>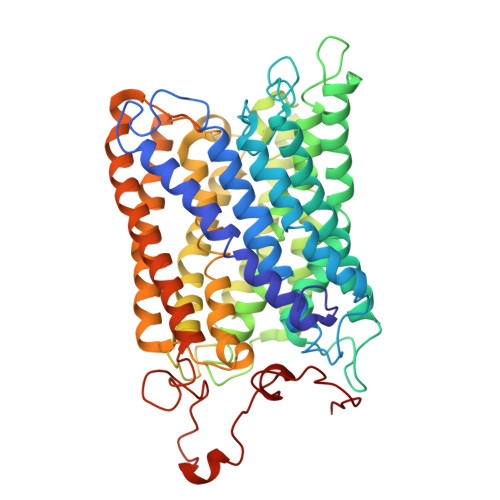 WLYSTNAKDIAVLYFMLAIFSGMAGTAMSLIIRLELAAPGSQYLHGNSQLFNVLVVGHAVLMIFFLVMPALIGGFGNYLLPLMIGATDTAFPRINNIAFWVLPMGLVCLVTSTLVESGAGTGWTVYPPLSSIQAHSGPSVDLAIFALHLTSISSLLGAINFIVTTLNMRTNGMTMHKLPLFVWSIFITAFLLLLSLPVLSAGITMLLLDRNFNTSFFEVSGGGDPILYEHLFWFFGHPEVYILIIPGFGIISHVVSTYSKKPVFGEISMVYAMASIGLLGFLVWSHHMYIVGLDADTRAYFTSATMIIAIPTGIKIFSWLATIHGGSIRLATPMLYAIAFLFLFTMGGLTGVALANASLDVAFHDTYYVVGHFHYVLSMGAIFSLFAGYYYWSPQILGLNYNEKLAQIQFWLIFIGANVIFFPMHFLGINGMPRRIPDYPDAFAGWNYVASIGSFIATLSLFLFIYILYDQLVNGLNNKVNNKSVIYNKAPDFVESNTIFNLNTVKSSSIEFLLTSPPAVHSFNTPAVQS> DCQQELSLVQTVTRGSRAFLSREEAQHFVKECGLLNCEAVLELLICHLRLGMEIMKLGRQLREAVRANDVDAMLKIAKEIIKVIGETGLDEVYRQLLKAAKEFLE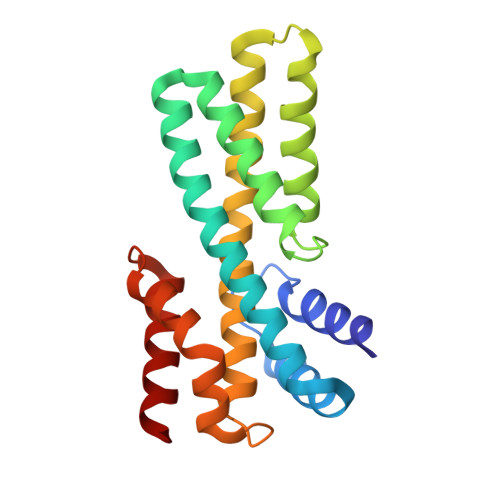RRAENFSHEEAVAFAQQIIQLIKQVECVQMRALGAVASLGCTDLLPQEHILLLTRPRLQELSAGSPGPVTNKATKILRHFEASC> EREALPPQKIEVLVLLPQDDSYLFSLTRVRPAIEYALRSVEGNGTGRRLLPPGT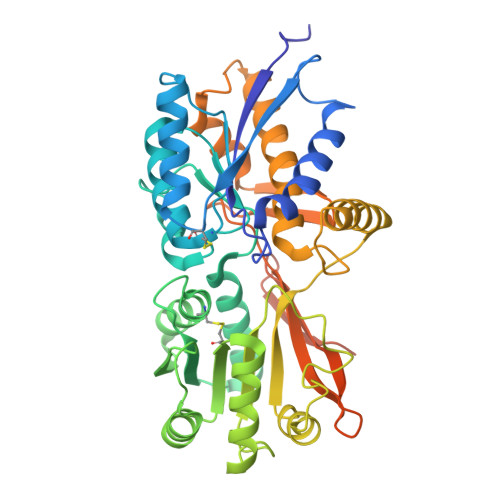RFQVAYEDSDCGNRALFSLVDRVAAARGAKPDLILGPVCEYAAAPVARLASHWDLPMLSAGALAAGFQHKDSEYSHLTRVAPAYAKMGEMMLALFRHHHWSRAALVYSDDKLERNCYFTLEGVHEVFQEEGLHTSIYSFDETKDLDLEDIVRNIQASERVVIMCASSDTIRSIMLVAHRHGMTSGDYAFFNIELFNSSSYGDGSWKRGDKHDFEAKQAYSSLQTVTLLRTVKPEFEKFSMEVKSSVEKQGLNMEDYVNMFVEGFHDAILLYVLALHEVLRAGYSKKDGGKIIQQTWNRTFEGIAGQVSIDANGDRYGDFSVIAMTDVEAGTQEVIGDYFGKEGRFEMRPNVKYPWGPLKLRIDENRIVEHTNSSPCKSCGLEESAVT>GSHMGTRTEIIRELERSLREQEELAKRLKELLRELE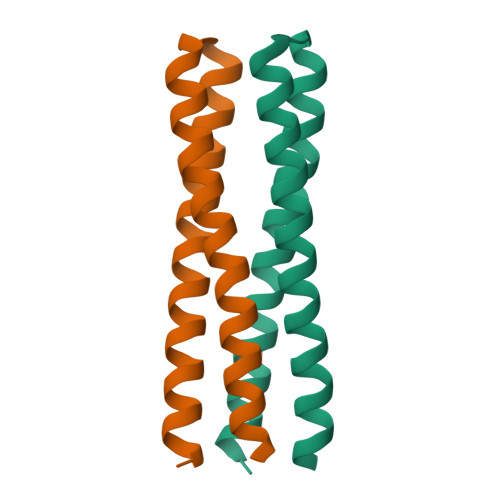RLQREGSSDEDVRELLREIKELVEEIEKLAREQKYLVEELKRQD[2x]2-hydroxy-6-(tetradecyloxy)benzoic acid | C21 H34 O4 | 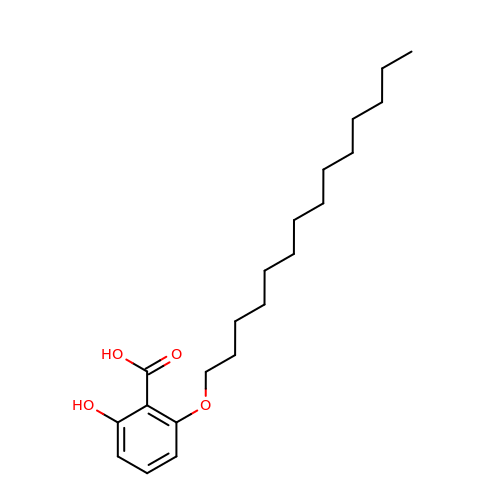COUQHIRIFUVLDU-UHFFFAOYSA-N> QAPSGWWLANIARQGRPAFNPDPNYKIFRNVKDYGAVGDGVTDDTAAINAAISDGNRCGQGCSSQTTTPALVYFPPGTYLVSKPIISYYYTQLVGDAISPPTLKAAANFEGMAVIDADPYDENGNNWWTNQNNFFRQVRNFVIDLTAMPFEVGSGIHWQVAQATSLQNIVFNMRTDGGDDNRQQGIFMDNGSGGLMVDLVFNGGRYGAFFGNQQFTTRNLTFNNCKTAIFMNWNWAWTFQDVKINNCEVGIDMSNGGPDGQTVGSVLLLDSHITNTGIGIKTAYDPAQPHTNGTLILDNVEMTGTPIAVQNDATGTTIVDGNQKIAFFAQGRTYGGSIGGTSGKAVQTTEQAIVKPNVLLDPATGKVFTRSRPQYEDVPVSSFVSVKANGAKGDGVTDDTDAIQAIFDSVTPEQIVYFDHGAYIITKTVRVPPNIRITGEALPLILAGGDSFFKDQANPKPVFQVGQPGERGRVEMSDLIFGTAGPQPGAIMMEWNVAGMEPGAAGLWDVHTRIGGYAGTQLELEQCAKNPNITNPIKPECFGSFLMLHVTPGGSAYLENTWYWVADHALEPEARDQQIDVFNGRGVLIEGDGPVWGWGTSSEHSVLHNYQFNNARNVFLALIQTETPYFQGNPDATQPFTVNPNFADPDFATSCTNSPNPEQCKRAWGVRAINSTDVFIYGAGLYSFFDNYDQECLKTQSCQTNMVSLEGNSQVHLFGLSTKA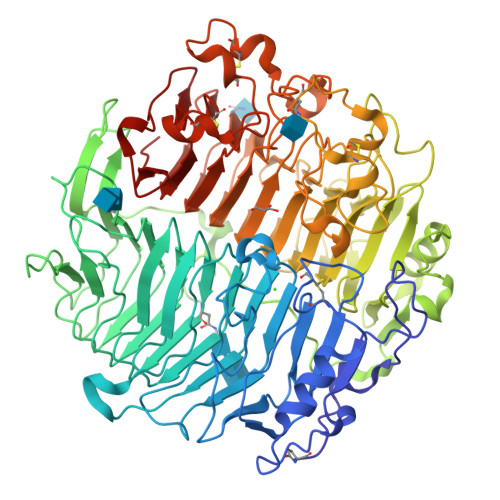SVNMLTVDGNAVALDADNRNNFCATVAWFQSTA>[2x]MAHHHHHHMSDIASHRESNGARSAQDERYARYPSLAGRAVLITGGATGIGASFVEHFARQGARVAFVDLDEQAARALAARLADAAHEPVFVACDLTDIAALRGAIEAIRARIGPIAALVNNAANDVRHAIADVTPDSFDACIAVNLRHQFFAAQAVIDDMKRLGGGSIVNLGSISWMLKNAGYPVYASAKAAVQGLTRALARELGPFGI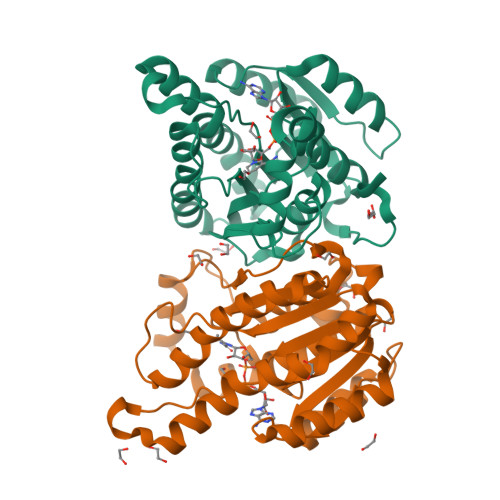RVNTLVPGWVMTDKQRRLWLDDAGRAAIKAGQCIDAELLPGDLARMALFLAADDSRMITAQDVVVDGGWA>GHMGTNRPLV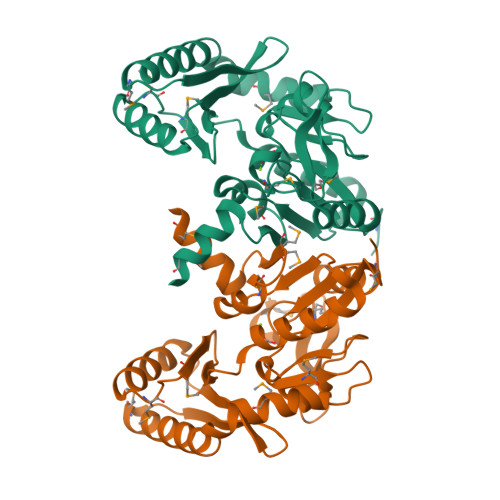FVDLDDTLFQTSRKMVEGTPRTTATLDVHGQPNGYMNPIQHSFISWLLASADVVPVTARDVEAYSRVKLPFTEGAICSHGGVMLHSDGSLDQDWHGQMAKSLWAFQDRLPALSEATLRIGKDMGYSLRGWVVEEEGLRHYVVTKQNESDDAVLSKVLAEVQARGMLEGMHIHANGNNLAFLPKGLAKRLAVQEWLRRDAKINGDRPVLGFGDSITDLGFMGLCHMWATPARSQLAKAVEEMII[2x]> NSLRACGPALMDMLRVACPNGFN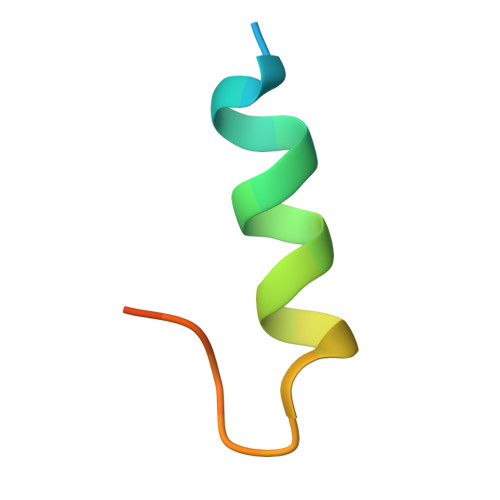SMFAK ETHYL PROPIONATE | C5 H10 O2 | 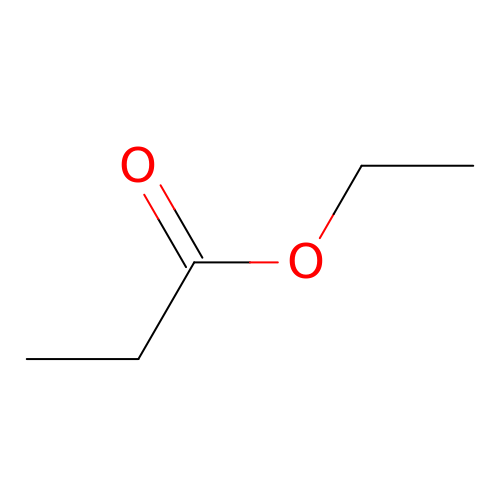FKRCODPIKNYEAC-UHFFFAOYSA-N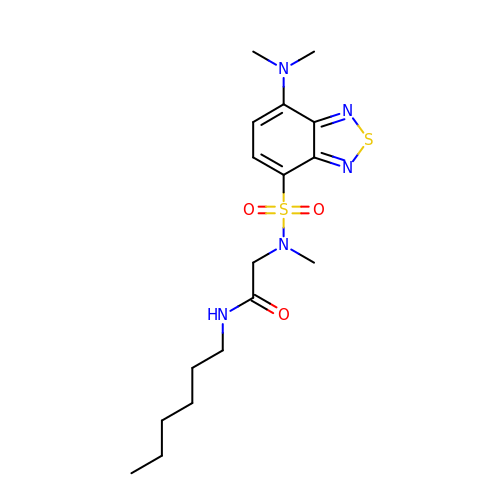N~2~-{[7-(dimethylamino)-2,1,3-benzothiadiazol-4-yl]sulfonyl}-N-hexyl-N~2~-methylglycinamide | C17 H27 N5 O3 S2 | YUOVTFFLGDNVBD-UHFFFAOYSA-N> GAACGACAAAGA;> CGTCGACTC;> TCTA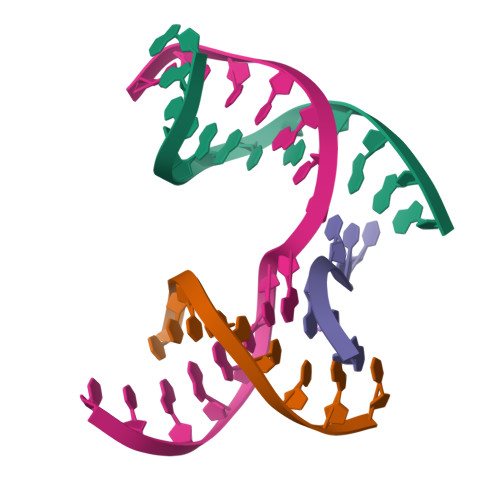CG;> TCGAGTCGTTGTCGT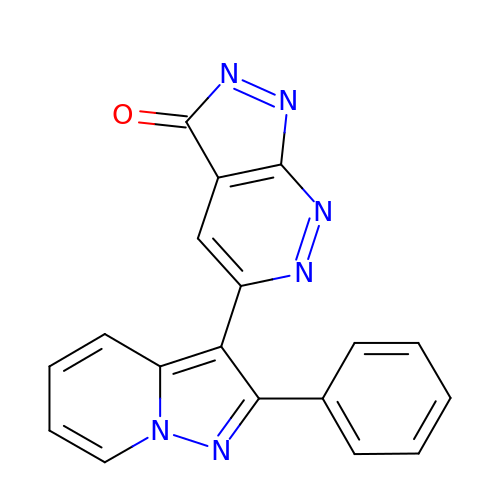5-(2-phenylpyrazolo[1,5-a]pyridin-3-yl)-3H-pyrazolo[3,4-c]pyridazin-3-one | C18 H10 N6 O | RURYGRIJIZXNQD-UHFFFAOYSA-N> MNSPISPIETVPVKLKPGMDGPKVKQWPLTEEKIKALVEICTEMEKEGKISKIGPENPYNTPVFAIKKKDSTKWRKLVDFRELNKRTQDFWEVQLGIPHPAGLKKNKSVTVLDVGDAYFSVPLDEDFRKYTAFTIPSINNETPGIRYQYNVLPQGWKGSPAIFQSSMTKILEPFRKQNPDIVIYQYMDDLYVGSDLEIGQHRTKIEELRQHLLRWGLTTPDKKHQKEPPFLWMGYELHPDKWTVQPIVLPEKDSWTVNDIQKLVGKLNWASQIYPGIKVRQLCKLLRGTKALTEVIPLTEEAELELAENREILKEPVHGVYYDPSKDLIAEIQKQGQGQWTYQIYQEPFKNLKTGKYARMRGAHTNDVKQLTEAVQKITTESIVIWGKTPKFKLPIQKETWETWWTEYWQATWIPEWEFVNTPPLVKLWYQLEKEPIVGAETFYVDGAANRETKLGKAGYVTNRGRQKVVTLTDTTNQKTELQAIYLALQDSGLEVNIVTDSQYALGIIQAQPDQSESELVNQIIEQLIKKEKVYLAWVPAHKGIGGNEQVDKLVSAGIRKVL;> MNSPISPIETVPVKLKPGMDGPKVKQWPLTEEKIKALVEICTEMEKEGKISKIGPENPYNTPVFAIKKKDSTKWRKLVDFRELNKRTQDFWEVQLGIPHPAGLKKNKSVTVLDVGDAYFSVPLDEDFRKYTAFTIPSINNETPGIRYQYNVLPQGWKGSP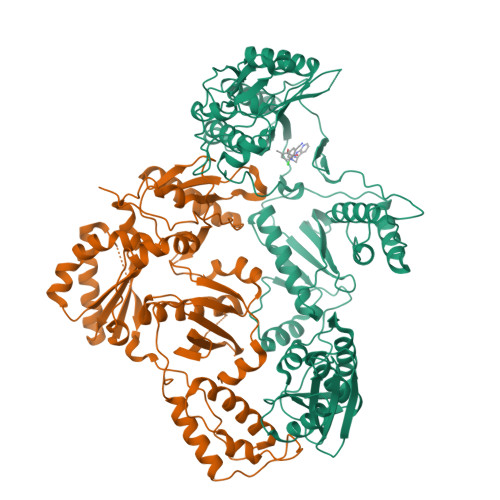AIFQSSMTKILEPFRKQNPDIVIYQYMDDLYVGSDLEIGQHRTKIEELRQHLLRWGLTTPDKKHQKEPPFLWMGYELHPDKWTVQPIVLPEKDSWTVNDIQKLVGKLNWASQIYPGIKVRQLCKLLRGTKALTEVIPLTEEAELELAENREILKEPVHGVYYDPSKDLIAEIQKQGQGQWTYQIYQEPFKNLKTGKYARMRGAHTNDVKQLTEAVQKITTESIVIWGKTPKFKLPIQKETWETWWTEYWQATWIPEWEFVNTPPLVKLWYQLEKEPIVGAETF>[4x]MASMTGGQQMGRGSEFMHHHHHHHHTATAETSTGTCVVLGQNQYGKAEVRLVKVTRNTARHEIQDLNVTSQLRGDFEAAHTAGDNAHVVATDTQKNTVYAFARDGFATTEEFLLRLGKHFTEGFDWVTGGRWAAQQFFWDRINDHDHAFSRNKSEVRTAVLEISGSEQAIVAGIEGLTVLKSTGSEFHGFPRDKYTTLQETTDRILATDVSARWRYNTVEVDFDAVYASVRGLLLKAFAETHSLALQQT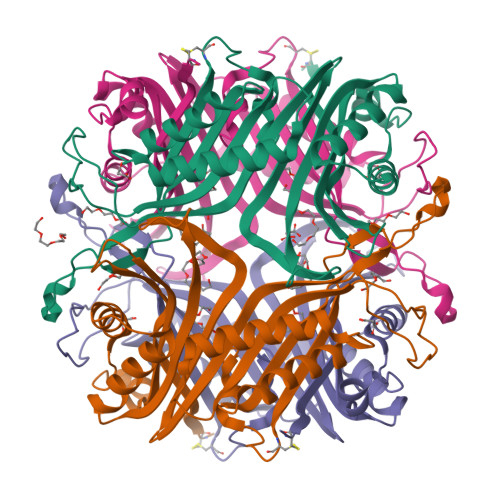MYEMGRAVIETHPEIDEIKMSLPNKHHFLVDLQPFGQDNPNEVFYAADRPYGLIEATIQRCGSRADHPIWSNIAGFC> GSHMIWEQHTVTLHRAPGFGFGIAISGGRDNPHFQSGETSIVISDVLKGGPAEGQLQENDRVAMVNGVSM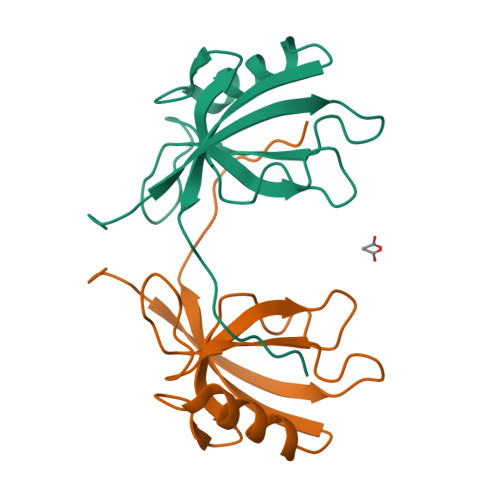DNVEHAFAVQQLRKSGKNAKITIRRKKGGGWRRTTYL RFCCtf18 is a seven‐subunit complex formed of Ctf18, Rfc2‐5 and the stable Dcc1‐Ctf8 sub‐complex. The complex is required for activation of the intra‐S‐phase checkpoint and proper establishment of sister chromatid cohesion. RFCCtf18 is a variant replication factor C‐like complex, the basic function of which is to load or unload a DNA sliding clamp in an ATP‐dependent manner 19, 20. Previous studies have shown that Dcc1 and Ctf8 are able to form a stable sub‐complex in vitro and that the C‐terminus of Ctf18 is required for the interaction with the Dcc1‐Ctf8 sub‐complex 39.

We identified a construct that expressed well in E. coli that includes the last 76 residues of Ctf18 (residues 666–741) with full‐length Dcc1 and Ctf8. Crystals of this complex (designated Ctf18C‐Dcc1‐Ctf8) were grown that diffracted to 2.4 Å resolution. The overall structure of Ctf18C‐Dcc1‐Ctf8 is extended and looks like a “hook”, as the C‐terminus of Dcc1 folds back towards Ctf8. The N‐terminus of Dcc1 from residues 1 to 115 forms a large heterodimer interface with Ctf8. The overall structure of the heterodimer resembles the “triple” β‐barrel fold which has previously been observed in RNase H2 53, and the transcription factors Rap30/74 54, Sfc1/7 55 and A49/34.5 56 (Fig EV2). Ctf18 binds as an extended peptide to a conserved groove present in the dimer interface of Dcc1‐Ctf8. The extreme C‐terminus of Ctf18 forms a short helix, which is partially buried in a hydrophobic pocket of the first “barrel” of Dcc1‐Ctf8. The structure shows that W736 and W740 make crucial contacts with other aromatic residues of both Dcc1 and Ctf8 as well as the extreme N‐terminal proline of Ctf8. The N‐terminal section of Ctf18 in our structure forms a beta sheet with Ctf8, with E724 from Ctf18 forming a salt bridge with R128 from Ctf8. Residues 666–713 of Ctf18 appear to be unstructured, suggesting they form a flexible linker between the Dcc1‐Ctf8 module and the rest of the Rfc1‐like domain of Ctf18.

>MSINLHSAPEYDPSYKLIQLTPELLDIIQDPVQNHQLRFKSLDKDKSEVVLCSHDKTWVLKQRKHSNTVLLMREFVPEQPITFDETLLFGLSKPYMDVVGFAKTESEFETRETHGELNLNSVPIYNGELDFSDKIMKRSSTKVIGTLEELLENSPCSALEGISKWHKIGGSVKDGVLCILSQDFLFKALHVLLMSAMAESLDLQHLNVEDTHHAVGKDIEDEFNPYTREIIETVLNKFAVQEQEAENNTWRLRIPFIAQWYGIQALRKYVSGISMPIDEFLIKWKSLFPPFFPCDIDIDMLRGYHFKPTDKTVQYIAKSTLPMDPKERFKVLFRLQSQWDLEDIKPLIEELNSRGMKIDSFIMKYARRKRLGKKTVVTSR[2x];>[2x]MPSVDIDASQWQKLTQSREKQTTVITPLGMMMLEIQGELELPKDFASLARRDSPNEGRFSEQDGETLIRFGSLQIDGERATLFVGKKQRLLGKVTKLDVPMGIMHFNSKDNKVELVDVMKYKVIFKDRPLPIM;>SGKVKTGLNSSSSTIDFFKNQYGLLKQTQELEETQKTIGSDETNQADDCNQTVKIWVKYNEGFSNAVRKNVTWNNLWE[2x]>[4x]ASVCFVKALYDYEGQTDDELSFPEGAIIRILNKENQDDDGFWEGEFNGRIGVFPSVLVEELSA;>[4x]KKPEIAQVIASYTA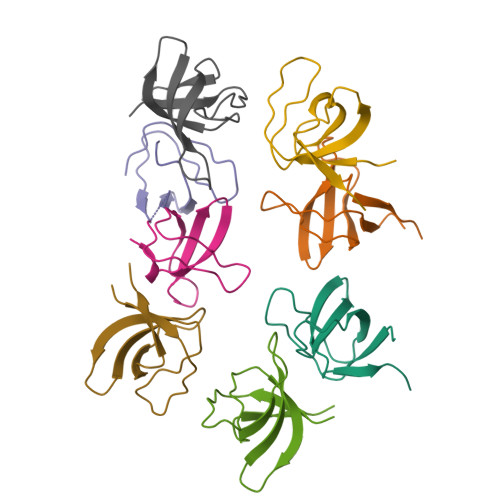TGPEQLTLAPGQLILIRKKNPGGWWEGELQARGKKRQIGWFPANYVKLLSP N~2~-1,3-BENZOXAZOL-2-YL-3-CYCLOHEXYL-N-{2-[(4-METHOXYPHENYL)AMINO]ETHYL}-L-ALANINAMIDE 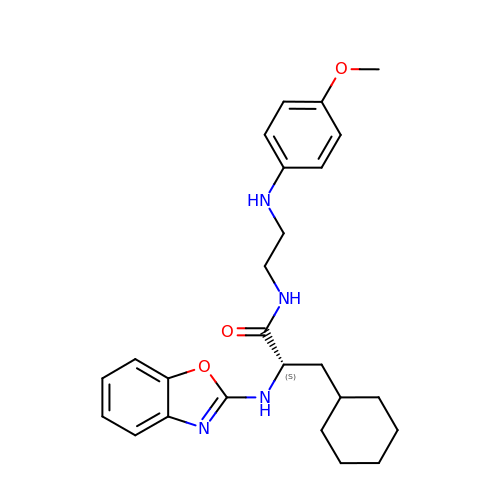| C25 H32 N4 O3 | VFNWTXUFNNOQHD-QFIPXVFZSA-N>GMPATKSLAELQAEVCRLDDRYLLERIIGAGSYGVVIRARDTKSDNRLVAMKRVNKEIFEEVILAKRILREIKLLAHFNDDNIIGLRNILTPEDPENFDHFYIVMDIMETD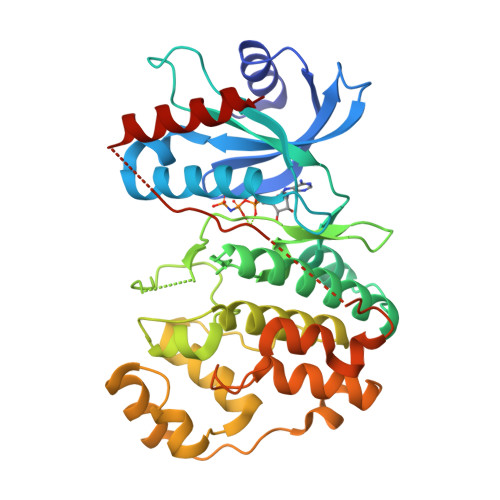LKQVLRSGQELTEAHIQFFIYQALRALHIIHSAGVIHRDITPANILVNTNCDLKICDFGLAKEENDQGEYMTDYVTMRWYRAPELVMEDKDYSAQIDVWGIGCILGELLGSRPLFQGKDRVNQLDKIVDVIGTPSEEDINSVGSSAAQKYLKKKSHRPQADWRQRYPTASPEALDLLRHMLVFNPKRRITVLQAMRHPFLEQLHDDADDNLSYALFRFDENEQKTIVDVKRAIYEESVKFHNE[2x]>[4x]MSLKLYGFSVSNYYNMVKLALLEKGLTFEE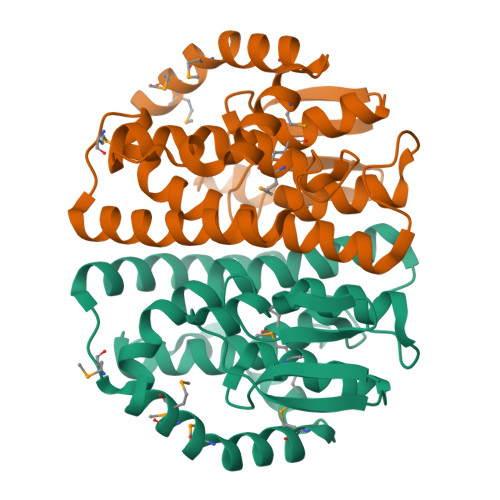VTFYGGQAPQALEVSPRGKVPVLETEHGFLSETSVILDYIEQTQGGKALLPADPFGQAKVRELLKEIELYIELPARTCYAESFFGMSVEPLIKEKARADLLAGFATLKRNGRFAPYVAGEQLTLADLMFCFSVDLANAVGKKVLNIDFLADFPQAKALLQLMGENPHMPRILADKEASMPAFMEMIRSGKREGHHHHHH>MTQMSDEQFRIFIETIKSLGPIKEEPPSKGSFSNCTVRFSGQRDHDAVDEFINAVETYKEVEGISDKDALKGLPLLFKSIAVVWWKGVRRDAKTWSDALQLLRDHFSPTKPSYQIYM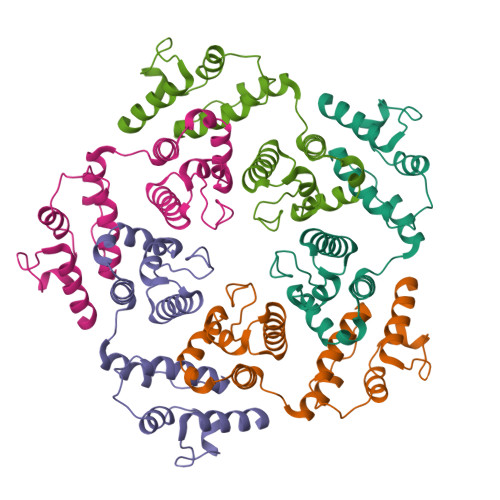EIFETKQSYDEVIDSFICKQRALLAKLPEGRHDEETELDFIYGLMQPKYRESIPRHEVKTFRELLDRGRTVERTRH[5x]5-(6-azanyl-4-chloranyl-1-propan-2-yl-pyrazolo[3,4-d]pyrimidin-3-yl)-1,3-benzoxazol-2-amine | C15 H14 Cl N7 O | 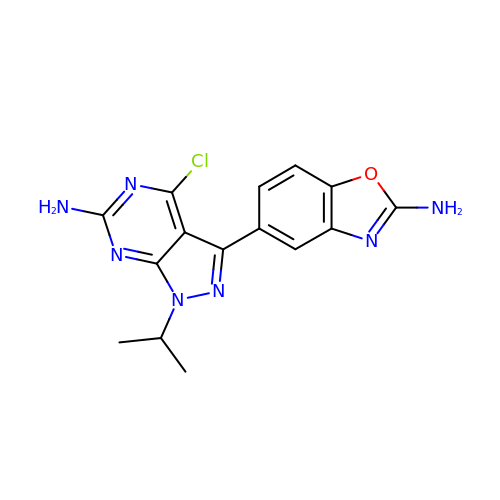YDFGZXSSYDSJRM-UHFFFAOYSA-N> GSMTAEEDMEDDTSWRSEATFQFTVERFSRLSESVLSPPCFVRNLPWKIMVMPRFYPDRPHQKSVGFFLQCNAESDSTSWSCHA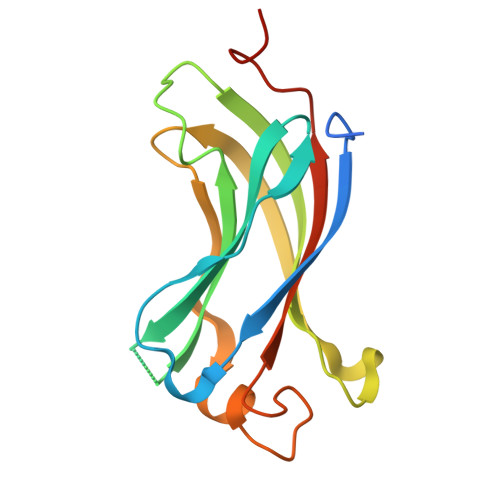QAVLKIINYRDDEKSFSRRISHLFFHKENDWGFSNFMAWSEVTDPEKGFIDDDKVTFEVFVQADAPHGVAWASTS(2R,3R)-2,3-dihydroxy-4-oxo-4-[(2R)-2-phenylpyrrolidin-1-yl]-N-(thiophen-2-ylmethyl)butanamide 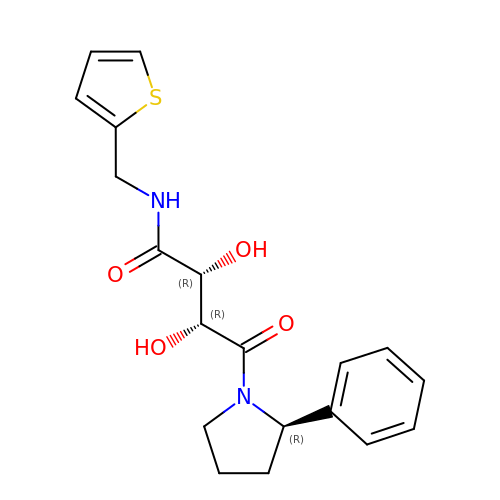| C19 H22 N2 O4 S | IJWSOCHVNGQZGZ-BRWVUGGUSA-N9-{(1R)-1-[(5P)-5-(4-chloro-1H-imidazol-2-yl)pyridin-3-yl]ethoxy}-1,4-dihydro-2H-pyrano[3,4-c]quinoline | C22 H19 Cl N4 O2 | 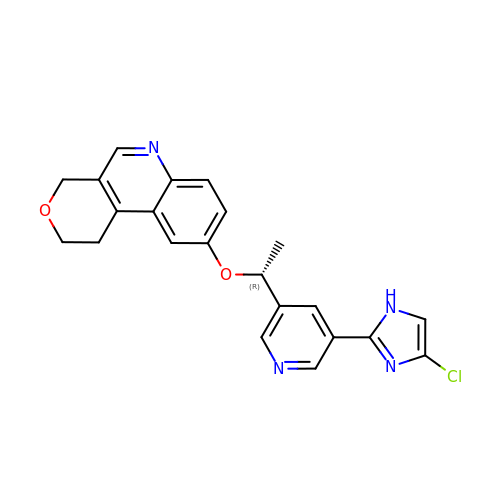ZZTIEDAGFODKQY-CYBMUJFWSA-N4-butyl-6-(1H-pyrrolo[2,3-b]pyridin-3-yl)pyrimidin-2-amine | C15 H17 N5 | 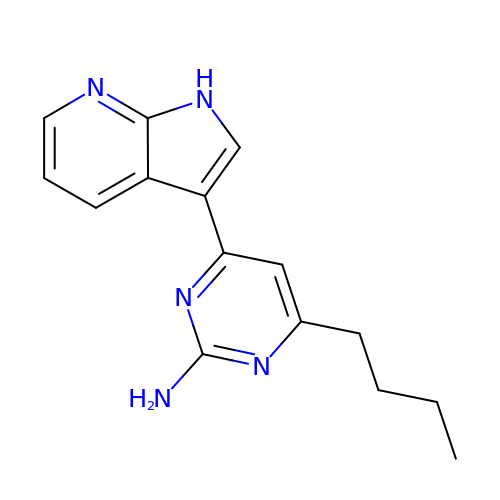JPZHGBZYRNZXPJ-UHFFFAOYSA-N>[4x]DTSSLIVEDAPDHVRPYVIRHYSHARAVTVDTQLYRFYVTGPSSGYAFTLMGTNAPHSDALGVLPHIHQKHYENFYCNKGSFQLWAQSGNETQQTRVLSSGDYGSVPRNVTHTFQIQDPDTEMTGVIVPGGFEDLFYYLGTNATDTTHTPYIPSSSDSSSTTGPDSSTISTLQ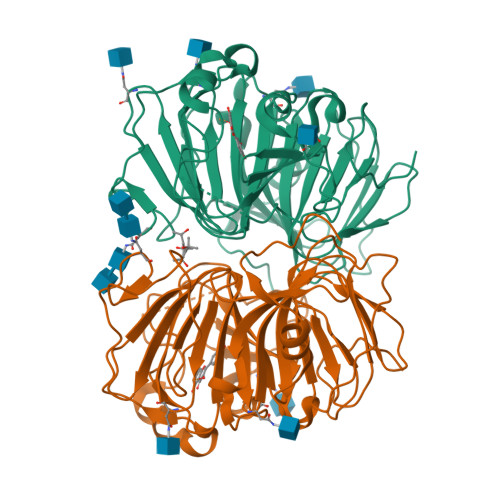SFDVYAELSFTPRTDTVNGTAPANTVWHTGANALASTAGDPYFIANGWGPKYLNSQYGYQIVAPFVTATQAQDTNYTLSTISMSTTPSTVTVPTWSFPGACAFQVQEGRVVVQIGDYAATELGSGDVAFIPGGVEFKYYSEAYFSKVLFVSSGSDGLDQNLVNGGEEWSSVSFPADW> SSPPVVDTVHGKVLGKFVSLEGFAQPVAIFLGIPFAKPPLGPLRFTPPQPAEPWSFVKNATSYPPMCTQDPKAGQLLSELFTNRKENIPLKLSEDCLYLNIYTPADLTKKNRLPVMVWIHGGGLMVGAASTYDGLALAAHENVVVVTIQYRLGIWGFFSTGDEHSRGNWGHLDQVAALRWVQDNIASFGGNPGSVTIFGESAGGESVSVLVLSPLAKNLFHRAISESGVALTSVLVKKGDVKPLAEQIAITAGCKTTTSAVMVHCLRQKTEEELLETTLKMKFLSLDLQGDPRESQPLLGTVIDGMLLLKTPEELQAERNFHTVPYMVGINKQEFGWLIPMQLMSYPLSEGQLDQKTAMSLLWKSYPLVCIAKELIPEATEKYLGGTDDTVKKKDLFLDLIADVMFGVPSVIVARNHRDAGAPTYMYEFQYRPSFSSDMKPKTVIGDHGDELFSVFGAPFLKEGASEEEIRLSKMVMKFWANFARNGNPNGEGLPHWPEYNQKEGYLQIGANTQAAQKLKDKEVAFWTNLFAK

Human carboxylesterase 1A (hCES1A) was employed as a target enzyme for inhibitory activity (IC50) screening due to its conservative catalytic serine residue. By the analysis of X-ray crystal structure, human CES1A has a serine esterase catalytic triad (Ser-221, His-468, and Glu-354), such catalytic triad is conserved in all mammalian species.. Herein, the halogen effects on the reactivity of the halogenated 2,2,2-trifluoroacetophenones as serine-targeting covalent warheads were investigated. Our results showed that introducing halogen atoms, especially Cl or Br, into the phenyl scaffold would influence the electron density around the ring, which led to different time-dependent inhibition response to the target serine hydrolase (hCES1A).

Surprisingly, dichloro-substituted analogues F-4 deriving from analogues F-1 and F-2 exhibited more promising contribution than monosubstituted analogues, but introducing three chloride atoms into the ring was not tolerated perhaps due to their enhanced passivation effect. The covalent interactions were evaluated by nano LC-MS/MS, which offered powerful evidence to support the formation of the covalent adducts and well-explained the time-dependent inhibition of these covalent fragments. Chloro-species compounds F-3 and F-4 were chosen to detect their covalent binding sites on hCES1A. Since the activity of electrophilic warheads and the formation of covalent adducts are related to temperature, we set the incubation conditions at two different temperature points (4 °C and 25°C, respectively). This analysis certainly found several allosteric binding sites, although no expected result of any compound covalently binding to Ser221 at the catalytic cavity of hCES1A. Successfully, the co-crystallography of hCES1A with F-3 and F-4 provided promising covalent binding modes at the catalytic triad. It could be obviously seen that the carbonyl group of F-4 was attacked by the oxygen of the OH group of Ser221, forming an expected hemiacetal covalent bond. The OH of the hemiacetal group introduced multiple hydrogen interactions with Gly143, Gly142 and Ala222 nearby, stabilising the formed hemiacetal adduct and favouring binding of the compound at this site. Notably, the co-crystallisation of the parent compound F and hCES1A failed to result in similar covalent interactions. This further proves that the halogen effect may promote the formation of covalent adducts by changing the sensitivity of the electrophilic warhead. The introduction of halogen atoms, particularly chlorine, into the phenyl scaffold enhances the benzocarbonyl reactivity in forming hemiacetal adducts with serine.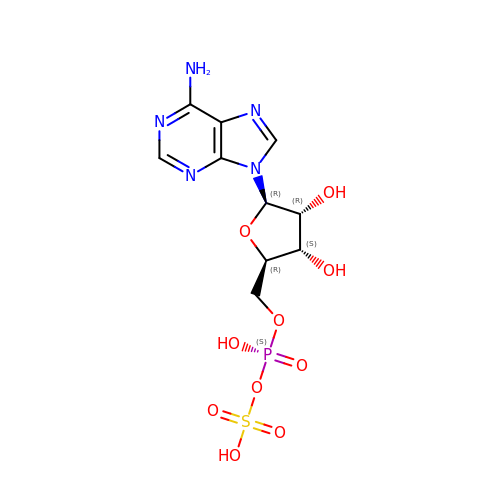ADENOSINE-5'-PHOSPHOSULFATE | C10 H14 N5 O10 P S | IRLPACMLTUPBCL-KQYNXXCUSA-N> TFDVGDEYEIIETIGNGAYGVVSSARRRLTGQQVAIKKIPNAFDVVTNAKRTLRELKILKHFKHDNIIAIKDILRPTVPYGEFKSVYVVLDLMESDLHQIIHSSQPLTLEHVRYFLYQLLRGLKYMHSAQVIHRDLKPSNLLVNENCELKIGDFGMARGLCTSPAEHQYFMTEYVATRWYRAPELMLSLHEYTQAIDLWSVGCIFGEMLARRQLFPGKNYVHQLQLIMMVLGT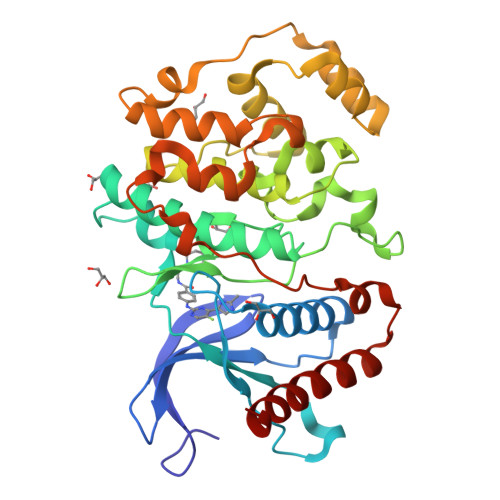PSPAVIQAVGAERVRAYIQSLPPRQPVPWETVYPGADRQALSLLGRMLRFEPSARISAAAALRHPFLAKYHDPDDEPDCAPPFDFAFDREALTRERIKEAIVAEIEDFHARREGI>[2x]MELESDPIAIVSMACRLPGGVNTPQRLWELLREGGETLSGFPTDRGWDLARLHHPDPDNPGTSYVDKGGFLDDAAGFDAEFFGVSPREAAAMDPQQRLLLETSWELVENAGIDPHSLRGTATGVFLGVAKFGYGEDTAAAEDVEGYSVTGVAPAVASGRISYTMGLEGPSISVDTACSSSLVALHLAVESLRKGESSMAVVGGAAVMATPGVFVDFSRQRALAADGRSKAFGAGADGFGFSEGVTLVLLERLSEARRNGHEVLAVVRGSALNQDGASNGLSAPSGPAQRRVIRQALESCGLEPGDVDAVEAHGTGTALGDPIEANALLDTYGRDRDAD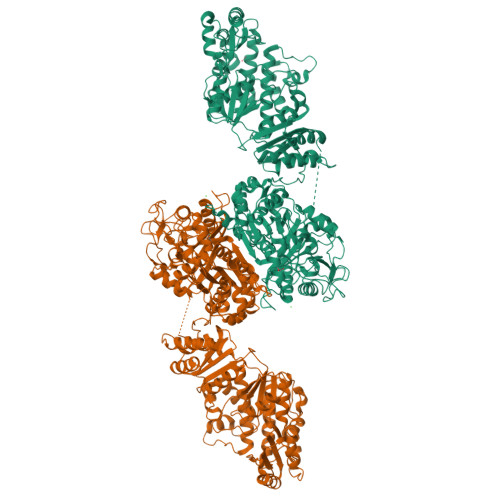RPLWLGSVKSNIGHTQAAAGVTGLLKVVLALRNGELPATLHVEEPTPHVDWSSGGVALLAGNQPWRRGERTRRAAVSAFGISGTNAHVIVEEAPEREHRETTAHDGRPVPLVVSARSTAALRAQAAQIAELLERPDADLAGVGLGLATTRARHEHRAAVVASTREEAVRGLREIAAGAATADAVVEGVTEVDGRNVVFLFPGQGSQWAGMGAELLSSSPVFAGKIRACDESMAPMQDWKVSDVLRQAPGAPGLDRVDVVQPVLFAVMVSLAELWRSYGVEPAAVVGHSQGEIAAAHVAGALTLEDAAKLVVGRSRLMRSLSGEGGMAAVALGEAAVRERLRPWQDRLSVAAVNGPRSVVVSGEPGALRAFSEDCAAEGIRVRDIDVDYASHSPQIERVREELLETTGDIAPRPARVTFHSTVESRSMDGTELDARYWYRNLRETVRFADAVTRLAESGYDAFIEVSPHPVVVQAVEEAVEEADGAEDAVVVGSLHRDGGDLSAFLRSMATAHVSGVDIRWDVALPGAAPFALPTYPFQRKRYWLQPAAPAAASDELAYRSSSVDKLAAALEHHHHHH>PGSEDENKLLEACIFKNNELLKNIQDVQSQISKIGLKDPTVPAVKHRKKSLIRLDKVLDEYEEEKRHLQEMANSLPHFKDGR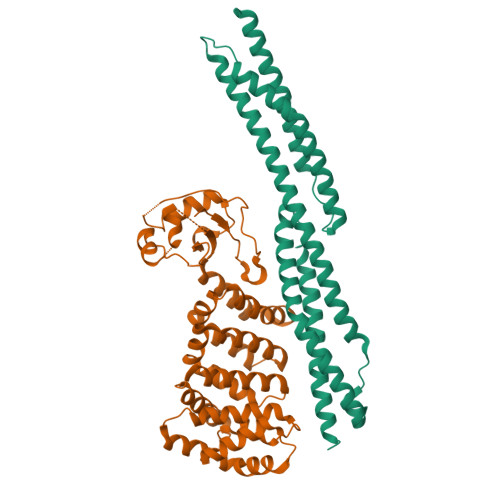EKTVNQQCQNTVVLWENTKALVTECLEQCGRVLELLKQYQNFKSILTTLIQKEESVISLQASYMGKENLKKRIAEIEIVKEEFNEHLEVVDKINQVCKNLQFYLNKMKTFEEPPFEKEANIIVDRWLDINEKTEDYYENLGRALALWD[2x];>SVVTVRVQYLEDTDPFACANFPEPRRAPTCSLDGALPLGAQIPAVHRLLGAPLKLEDCALQVSPSGYYLDTELSLEEQREMLEGFYEEISKGRKPTLILRTQLSVRVNAILEKLYSSSGPELRRSLFSLKQIFQEDKDLVPEFVHSEGLSCLIRVGAAADHNYQSYILRALGQLMLFVDGMLGVVAHSDTIQWLYTLCASLSRLVVKTALKLLLVFVEYSENNAPLFIRAVNSVASTTGAPPWANLVSILEEKNGADPELLVYTVTLINKTLAALPDQDSFYDVTDALEQQGMEALVQRHLGTAGTDVDLRTQLVLYENAL[2x]>[8x]MKIKQVHVRASKIKLKETFTIALGTIESADSAIVEIETEEGL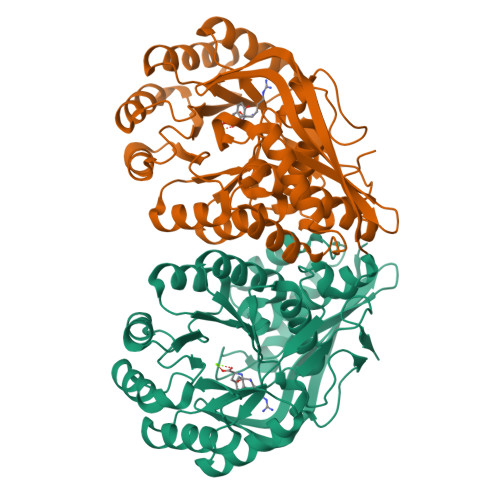VGYGEGGPGIFITGETLAGTLETIELFGQAIIGLNPFNIEKIHEVMDKISAFAPAAKAAIDIACYDLMGQKAQLPLYQLLGGYDNQVITDITLGIDEPNVMAQKAVEKVKLGFDTLKIKVGTGIEADIARVKAIREAVGFDIKLRLDANQAWTPKDAVKAIQALADYQIELVEQPVKRRDLEGLKYVTSQVNTTIMADESCFDAQDALELVKKGTVDVINIKLMKCGGIHEALKINQICETAGIECMIGCMAEETTIGITAAAHLAAAQKNITRADLDATFGLETAPVTGGVSLEAKPLLELGEAAGLGISH>[2x]GLPARSSSISNTNRTGENPMITPIISSNLGLKHRVTLRKATLASLMQSLSGESSNRVMWNDRYDTLLIARDPREIKNAIEKSVTDFGGLENYKELTGGADPFALMTPVCGLSANNIFKLMTEKDVPIDPTSIEYLENTSFAEHVNTLDSHKNYVVIVNDGRLGHKFLIDLPALTQGPRTAYIIQSDLGGGALPAVRVEDWISRRGSDPVSLDELNQLLSKDFS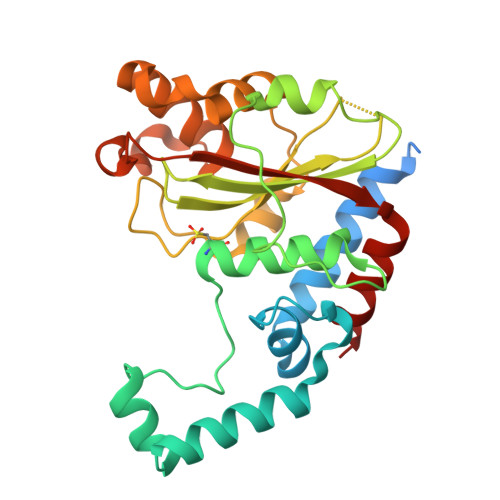KMPDDVQTRLLASILQIDKDPHKVDIKKLHLDGKLRFASHEYDFRQFQRNAQYVAGLG Entrectinib | C31 H34 F2 N6 O2 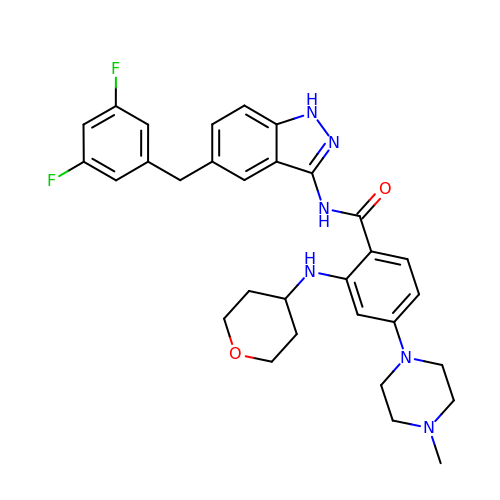| HAYYBYPASCDWEQ-UHFFFAOYSA-N>GPAMEKYEGDWVNGKMHGHGKYIYSDGGVYEGDWIDGKMHGKGTYVFPNGNVYEGEWAHDMKDGYGVLTYQNGEKYEGYWKQDKVHGKGTLTYTRGDKYIGDWMDAKKDGEGELIYANGDRFKGQWADDRANGFGVFTYANGNRYEGEWTDDKRHGRGVFYCAEDGSAYEGEFVGGRKEGN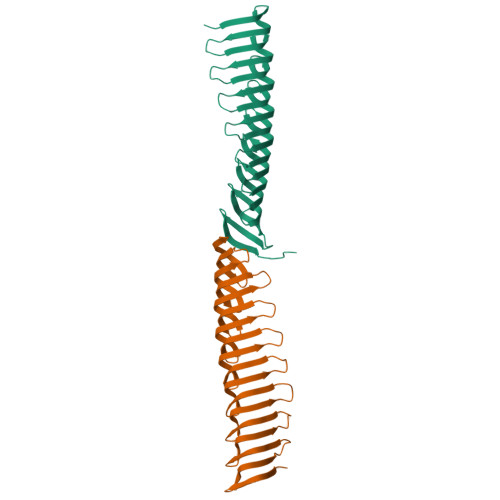GILRLATGHQLEGTWSGGQLVRVTSFVFAQDSPWLNVDL[2x]(METHYLPYRIDAZINE PIPERIDINE BUTYLOXYPHENYL)ETHYLACETATE | C23 H31 N3 O3 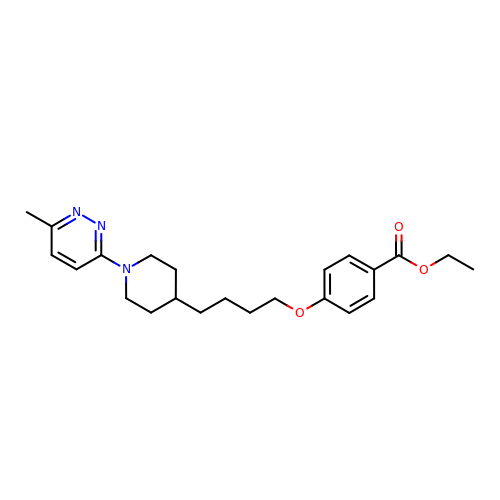| AQILFLLHLFBLLG-UHFFFAOYSA-N>MNLIPTVIETTNRGERAYDIYSRLLKDRIIMLGSQIDDNVANSIVSQLLFLQAQDSEKDIYLYINSPGGSVTAGFAIYDTIQHIKPDVQTICIGMAASMGSFLLAAGAKGKRFALPNAEVMIHQPLGGAQGQATEIEIAANHILKTREKLNRILSERTGQSIEKIQQDTDR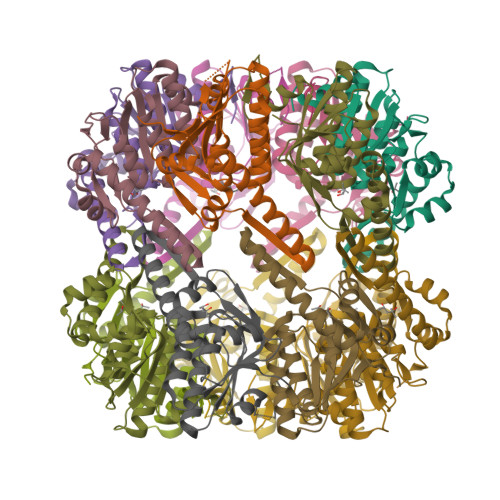DNFLTAAEAKEYGLIDEVMEPEHHHHHH[14x]>[3x]GAEIYNKDGNKVDLYGKAVGLHYFSKGNGENSYGGNGDMTYARLGFKGETQINSDLTGYGQWEYNFQGNNSEGADAQTGNKTRLAFAGLKYADVGSFDYGRNYGVVYDALGYTDMLPEFGGDTAYSDDFFVGRVGGVATYRNSNFFGLVDGLNFAV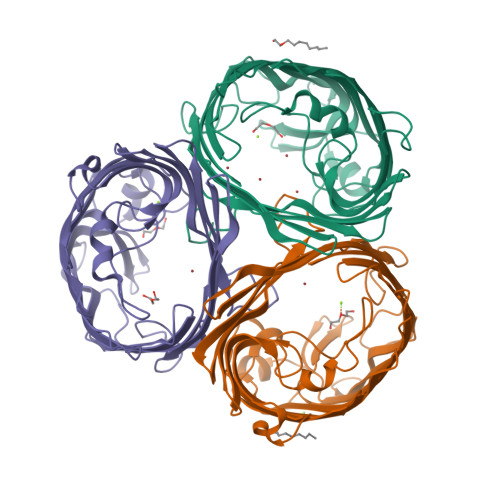QYLGKNERDTARRSNGDGVGGSISYEYEGFGIVGAYGAADRTNLQEAQPLGNGKKAEQWATGLKYDANNIYLAANYGETRNATPITNKFTNTSGFANKTQDVLLVAQYQFDFGLRPSIAYTKSKAKDVEGIGDVDLVNYFEVGATYYFNKNMSTYVDYIINQIDSDNKLGVGSDDTVAVGIVYQF>[2x]MATVLTKGEIVLFALRKFAIASNASLTDVEPQSIEDGVNDLEDMMSEWMINPGDIGYAFATGDEQPLPDDESGLPRKYKHAVGYQLL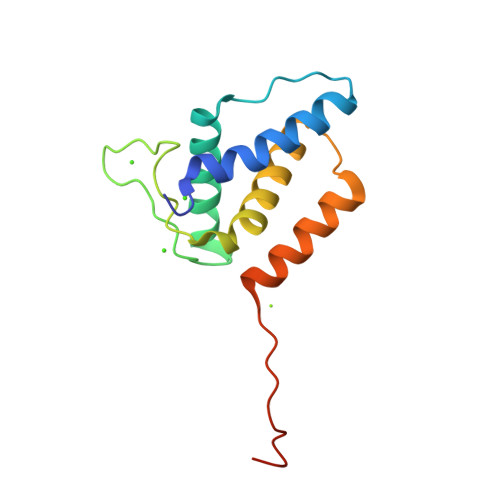LRMLSDYSLEPTPQVLSNAQRSYDALMTDTLVVPSMRLEHHHHHH> CQFALKQPQEKIVPYVRQPEEIIHGRPLFFATAVTFAGFGVGLLVESHEGRPTKIEGNPDHPASLGSTDLITQAMILTMYDPDRSQAPTNAGQETTWDAFVAAATAAMQAQTAKQGAGLRVLSGSLTSPTLIAQKQQLLTQFPQAKWYEYEPVGRDNANAGARLAFGADVHTIYRLDTAKVIVGFDADFTAPSPTGVRMARQLADGRRIRKGTKEVNRLYLAESTPSITGLLADHRLPVRSSQIEHLVRALATLVGVPNVAAGAPLSDTEKKWVEAAAKDLQANRGACVVLVGESQPPVVHALGHAINAQLGNVGSTVVYTEPVEDDPSGGIAALSALTQEMNAGTVEVLLMIESNPVYNAPADIPFAEALAKVPLSMHVGLYRDETAQQSVWHINGAHFLEAWGDVRAFDGTTTIVQPLIAPLYNGKSAIEVLNVLLGKPQETGYQTLTAYWQTQDASGNFRVFWNTALHDGVITATQARSRQVTLQQGFADAAPPAPTQGLEIVFRPDPSLWDGAFANNAWLQETPKPYTKLTWDNVALMSVRTANALGLKNGDVVRLTYQGRSVDAPVWVQPGHADDSVTVHFGFGRTAAGRVGNNVGFNAYRLRTSATPWFGVGLEVAKVGENYKLASTQGHFLMEGRKKDLVRYGTLAEYVEDEKFLQVEKEEPISLIGEYEYNGYKWGMSIDLNVCNSCNACVVACQSENNIPVVGKDEVWLGREMHWIRIDQYYVGDEHTPNVYNMVMLCQQCEHAPCEIVCPVAATVHDAEGLNNMVYNRCVGTKYCSNNCPYKVRRFNFLQYQDVPYRSPIDASTENDSIPVLKMMRNPDVTVRARGVMEKCTFCVQRINEARIQARTENRRIADGEIMTACQQVCP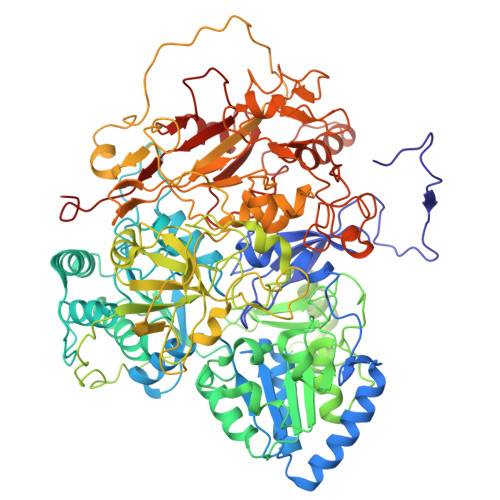TQAIVFGDLNDPQARVVDLKEQPLKYTSLDKLNTKPRVSYLAKIKNLNPDLAEEKTA>[6x]PESPSKLASAIQKAHEEGICGIRSVTRLENLMWKQITPELNHILTENEVKLTIMTGDIKGIMQAGKRSLRPQPTELKYSWKAWGKAKMLSTELHNHTFLIDGPETAECPNTNRAWNSLEVEDYGFGVFTTNIWLKLKERQDVFCDSKLMSAAIKDNRAVHADMGYWIESALNDTWKIEKASFIEVKSCHWPKSHTLWSNGVLESEMIIPKNFAGPVSQHNYRPGYHTQTAGPWHLGRLEMDFDFCEGTTVVVTEDCGNRGPSLRTTTASGKLITEWCCRSCTLPPLRYRGEDGCWYGMEIRPLKEK

NS1 is secreted alongside dengue virus particles during an infection. It is a multifunctional protein which exists in different oligomeric forms intracellularly and extracellularly, and they play distinctly different roles. The intracellular NS1 (iNS1), exists as a membrane associated dimeric form and is a part of the viral replication complex. The extracellular secreted NS1 (sNS1), exists in higher oligomeric forms. sNS1 likely causes vascular leakage symptoms in DHF/DSS via two pathways—indirectly, by stimulating the innate immune response through activation of complement and Toll-like receptors, and directly, by binding to endothelial cells causing endothelial hyperpermeability. sNS1 when bound directly to endothelial cells causes barrier dysfunction of the cell monolayer as demonstrated in an in vitro trans-endothelial electrical resistance (TEER) assay. Here we show by cryoEM that the recombinant sNS1 exists in multiple oligomeric states: the tetrameric (stable and loose conformation) and hexameric structures.

Only a minority of the recombinant sNS1 population is hexameric and this cryoEM structure was determined to 8 Å resolution. For the hexamers, since we only had a limited number of particles (~30,000 particles), we performed only non-uniform refinement with D3 symmetry imposed and obtained an 8 Å map. The low-resolution structure suggests that the NS1 molecules in the hexameric state are interacting loosely with each other. Fitting of iNS1 suggests that three dimers interact with each other via their wing domain and the distal end of the β-ladder. This interaction is similar to that in the loose tetramer. The density in the central core of the hexamer is weak and we were therefore unable to determine if the dimers have a β-roll or elongated β-sheet conformation. The two neighboring dimers in the stable and loose tetramers have a total buried area of ~650–690 Å2, compared to that in the hexamer 307 Å2. All epitopes in the hexamer are partially exposed (37.5%).> TTIVSVRRNGHVVIAGDGQAT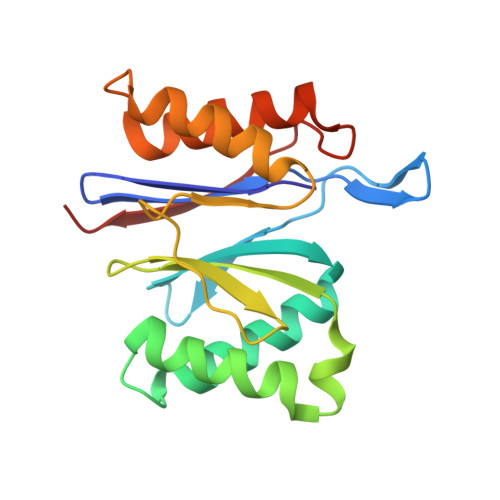LGNTVMKGNVKKVRRLYNDKVIAGFAGGTADAFTLFELFERKLEMHQGHLVKAAVELAKDWRTDRMLRKLEALLAVADETASLIITGNGDVVQPENDLIAIGSGGPYAQAAARALLENTELSAREIAEKALDIAGDICIYTNHFHTIEELSYKA[(2R,3S,4R,5R)-5-(6-amino-9H-purin-9-yl)-3,4-dihydroxytetrahydrofuran-2-yl]methyl (2R)-1-{(2S,3S,4R,5S,6R)-6-[(1S)-1,2-dihydroxyethyl]-3,4,5-trihydroxytetrahydro-2H-pyran-2-yl}propan-2-yl 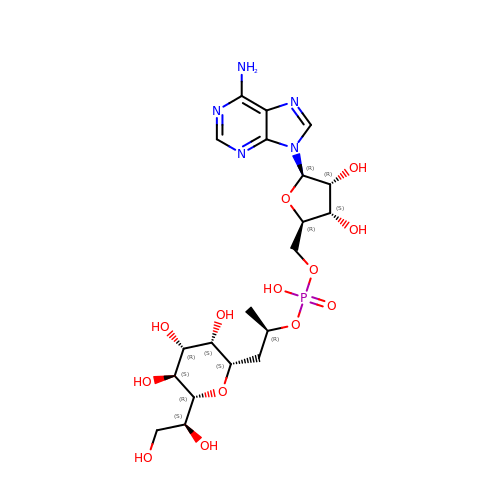hydrogen (R)-phosphate (non-preferred name) | C20 H32 N5 O13 P | KMYAQBXCNBRSNR-VHKXYEKJSA-N> MGGSEVGTVPVTWRLGVDVGERSIGLAAVSYEEDKPKEILAAVSWIHDGGVGDERSGASRLALRGMARRARRLRRFRRARLRDLDMLLSELGWTPLPDKNVSPVDAWLARKRLAEEYVVDETERRRLLGYAVSHMARHRGWRNPWTTIKDLKNLPQPSDSWERTRESLEARYSVSLEPGTVGQWAGYLLQRAPGIRLNPTQQSAGRRAELSNATAFETRLRQEDVLWELRCIADVQGLPEDVVSNVIDAVFCQKRPSVPAERIGRDPLDPSQLRASRACLEFQEYRIVAAVANLRIRDGSGSRPLSLEERNAVIEALLAQTERSLTWSDIALEILKLPNESDLTSVPEEDGPSSLAYSQFAPFDETSARIAEFIAKNRRKIPTFAQWWQEQDRTSRSDLVAALADNSIAGEEEQELLVHLPDAELEALEGLALPSGRVAYSRLTLSGLTRVMRDDGVDVHNARKTCFGVDDNWRPPLPALHEATGHPVVDRNLAILRKFLSSATMRWGPPQSIVVELARGASESRERQAEEEAARRAHRKANDRIRAELRASGLSDPSPADLVRARLLELYDCHCMYCGAPISWENSELDHIVPRTDGGSNRHENLAITCGACNKEKGRRPFASWAETSNRVQLRDVIDRVQKLKYSGNMYWTRDEFSRYKKSVVARLKRRTSDPEVIQSIESTGYAAVALRDRLLSYGEKNGVAQVAVFRGGVTAEARRWLDISIERLFSRVAIFAQSTSTKRLDRRHHAVDAVVLTTLTPGVAKTLADARSRRVSAEFWRRPSDVNRHSTEEPQSPAYRQWKESCSGLGDLLISTAARDSIAVAAPLRLRPTGALHEETLRAFSEHTVGAAWKGAELRRI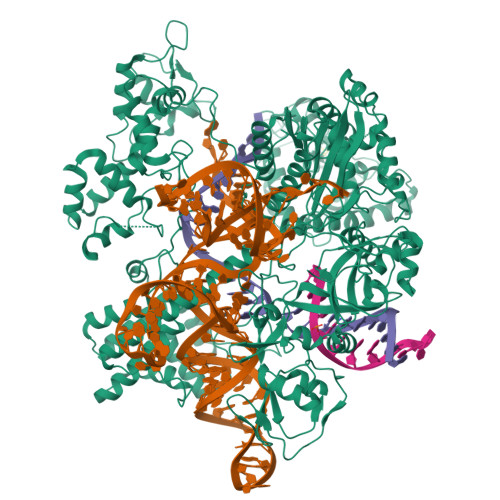VEPEVYAAFLALTDPGGRFLKVSPSEDVLPADENRHIVLSDRVLGPRDRVKLFPDDRGSIRVRGGAAYIASFHHARVFRWGSSHSPSFALLRVSLADLAVAGLLRDGVDVFTAELPPWTPAWRYASIALVKAVESGDAKQVGWLVPGDELDFGPEGVTTAAGDLSMFLKYFPERHWVVTGFEDDKRINLKPAFLSAEQAEVLRTERSDRPDTLTEAGEILAQFFPRCWRATVAKVLCHPGLTVIRRTALGQPRWRRGHLPYSWRPWSADPWSGGTP4-FLUOROBENZENESULFONAMIDE | C6 H6 F N O2 S | 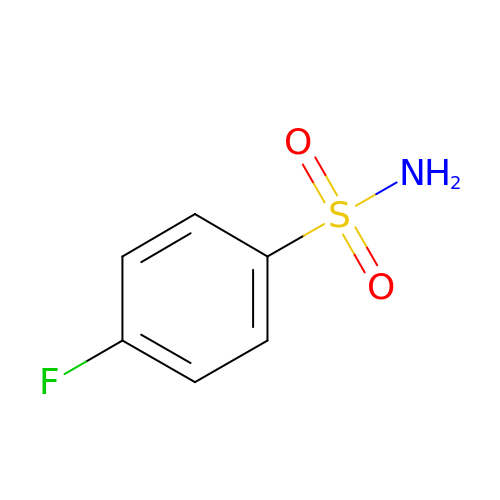LFLSATHZMYYIAQ-UHFFFAOYSA-N> PKALIVYGSTTGNTEYTAETIARELADAGYEVDSRDAASVEAGGLFEGFDLVLLGCSTWGDDSIE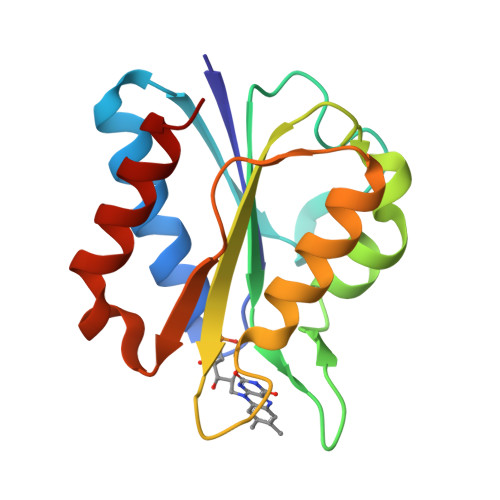LQDDFIPLFDSLEETGAQGRKVACFGCGDSSWEYFCGAVDAIEEKLKNLGAEIVQDGLRIDGDPRAARDDIVGWAHDVRGAI> ADYDLKFGMNAGTSSNEYKAAEMFAKEVKEKSQGKIEISLYPSSQLGDDRAMLKQLKDGSLDFTFAESARFQLFYPEAAVFALPYVISNYNVAQKALFDTEFGKDLIKKMDKDLGVTLLSQAYNGTRQTTSNRAINSIADMKGLKLKVPNAATNLAYAKYVGASPTPMAFSEVYLALQTNAVDGQENPLAAVQAQKFYEVQKFLAMTNHILN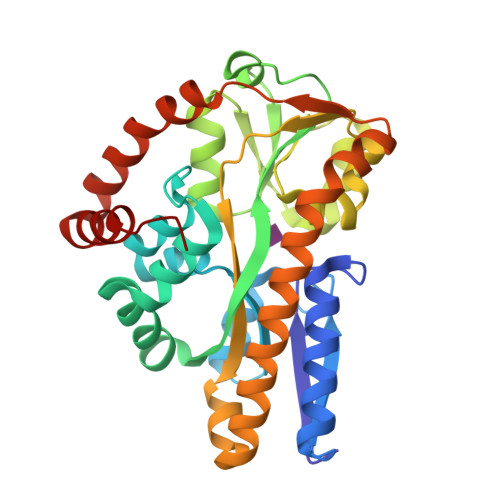DQLYLVSNETYKELPEDLQKVVKDAAENAAKYHTKLFVDGEKDLVTFFEKQGVKITHPDLVPFKESMKPYYAEFVKQTGQKGESALKQIEAINPHH>[2x]GSHMSRKIRDLIESKRFQNVITAIIVLNGAVLGLLTDTTLSASSQNLLERVDQLCLTIFIVEISLKIYAYGVRGFFRSGWNLFDFVIVAIALMPAQGSLSVLRTFRIFRVMRLVSVIPTMRRVVQGMLLALPGVGSVAALLTVVFYIAAVMATNLYGATFPEWFGDLSKSLYTLFQVMTLESWSMGIVRPVMNVHPNA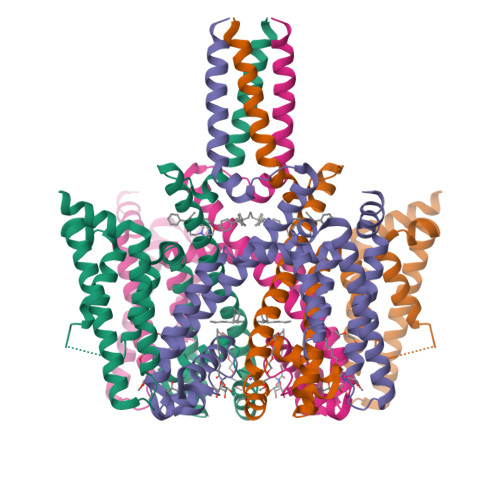WVFFIPFIMLTTLTVLNLFIGIIVDAMAITKEQEEEAKTGHHQEPISQTLLHLGDRLDRIEKQLAQNNELLQRQQPQKK>MNSQLTLRALERGD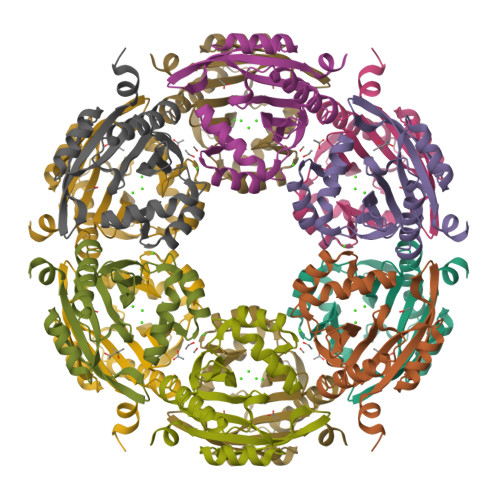LRFIHNLNNNRNIMSYWFEEPYESFDELEELYNKHIHDNAERRFVVEDAQKNLIGLVELIEINYIHRSAEFQIIIAPEHQGKGFARTLINRALDYSFTILNLHKIYLHVAVENPKAVHLYEECGFVEEGHLVEEFFINGRYQDVKRMYILQSKYLNRSE[3x]>[4x]GPTPEAPYASLTEIEHLVQSVCKSYRETCQLRLED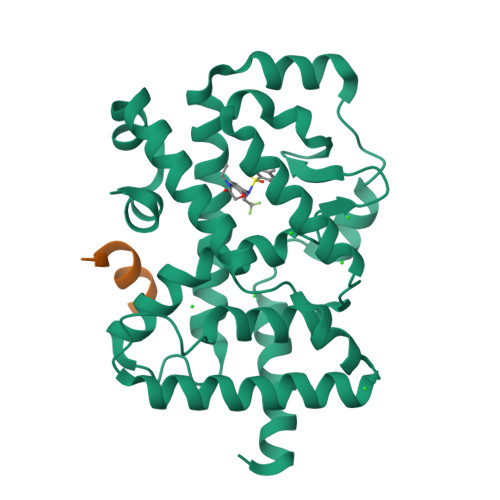LLRQRSNIFSREEVTGYQRKSMWEMWERCAHHLTEAIQYVVEFAKRLSGFMELCQNDQIVLLKAGAMEVVLVRMCRAYNADNRTVFFEGKYGGMELFRALGCSELISSIFDFSHSLSALHFSEDEIALYTALVLINAHRPGLQEKRKVEQLQYNLELAFHHHLCKTHRQSILAKLPPKGKLRSLCSQHVERLQIFQHLHPIVVQAAFPPLYKELFSTTETESPVGLSK;>[4x]EFPYLLSLLGEVSPQ>[2x]MTDLKASSLRALKLMHLATANDDDTDEKVIA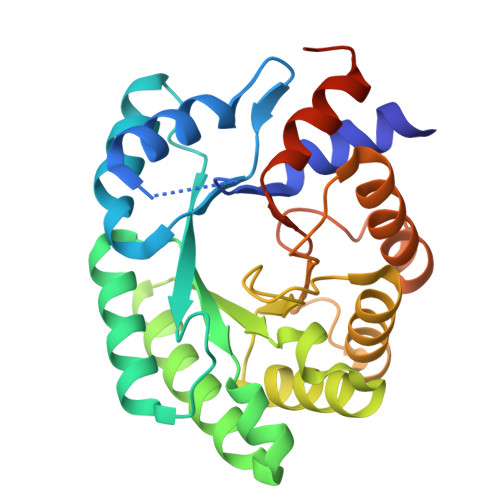LCHQAKTPVGTTDAIYIYPRFIPIARKTLKEQGTPEIRIWTSTNFPHGNDDIDIALAETRAAIAYGADGVAVVFPYRALMAGNEQVGFDLVKACKEACAAANVLLSVIIETGELKDEALIRKASEISIKAGADHIVTSTGKVAVGATPESARIMMEVIRDMGVEKTVGFIPAGGVRTAEDAQKYLAIADELFGADWADARHYAFGASSLLASLLKALGHGDGKSASSYGSLE> LWMHKVPASLMVSLGEDAHFQCPHNSSNNANVTWWRVLHGNYTWPPEFLGPGEDPNGTLIIQNVNKSHGGIYVCRVQEGNESYQQSCGTYLRVRQPPPRPFLDMGEGTKNRIITAEGIILLFCAVVPGTLLLFRKRW;>[2x]LPPKVSVFVPPRDGFFGNPRKSKLICQATGFSPRQIQVSWLREGKQVGSGVTTDQVQAEAKESGPTTYKVTSTLTIKESDWLGQSMFTCRVDHRGLTFQQNASSMCVPDQDTAIRVFAIPPSFASIFLTKSTKLTCLVTDLTTYDSVTISWTRQNGEAVKTHTNISESHPNATFSAVGEASICEDDWNSGERFTCTVTHTDLPSPLKQTISRPKGVALHRPDVYLLPPAREQLNLRESATITCLVTGFSPADVFVQWMQRGQPLSPEKYVTSAPMPEPQAPGRYFAHSILTVSEEEWNTGETYTCVVAHEALPNRVTERTVDKSTEGEVSADEEGFENLWAT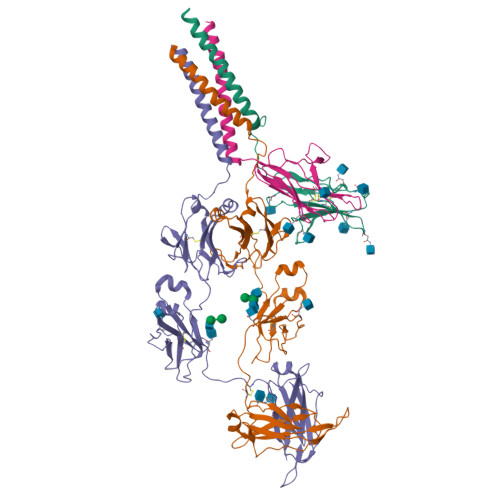ASTFIVLFLLSLFYSTTVTLFK;> SRIWQSPRFIARKRGFTVKMHCYMNSASGNVSWLWKQEMDENPQQLKLEKGRMEESQNESLATLTIQGIRFEDNGIYFCQQKCNNTSEVYQGCGTELRVMGFSTLAQLKQRNTLKDGIIMIQTLLIILFIIVPIFLLLD>[2x]XKKLLKCLKCLLX

Herein we report the first X-ray crystal structures of mixed chirality α-helices in short peptides comprising only natural residues as the example of a stapled bicyclic and a linear membrane disruptive amphiphilic antimicrobial peptide (AMP) containing seven l- and four d-residues, as complexes of fucosylated analogs with the bacterial lectin LecB. The mixed chirality α-helices are superimposable onto the homochiral α-helices and form under similar conditions as shown by CD spectra and MD simulations but non-hemolytic and resistant to proteolysis. To get a direct insight into the structure of AMBP bp65/bp69 and their linear analogs ln65/ln69, we performed several crystallization studies using either the compounds themselves or their racemates to be crystallized as pure compounds, or their fucosylated derivatives of both mirror image peptides as complexes with the P. aeruginosa lectin LecB. While previous reports of similar mixed chirality AMPs concluded on either unordered conformations or helical conformations appearing in a membrane environment based on deconvolution of FTIR spectra, here we reported X-ray crystallographic evidence of short mixed chirality helices consisting of only natural residues existing as helix bundles within the protein environment of a lectin and almost perfectly superimposable with their parent homochiral α-helices. These direct observations unequivocally demonstrate that the α-helical fold with only natural residues can sometimes tolerate multiple stereochemical inversions without significant conformational changes.

Herein we report that optimization of bp3 by sequence and residue chirality variations followed by structural studies led us to the first X-ray crystal structure of an AMPB in the form of bp65. The structure of bp65 features an α-helical fold essentially identical to that of the corresponding linear peptide ln65 but comprising a bicyclic helix staple. In all four individually resolved homochiral bicyclic structures, the peptides were present in almost perfectly superimposable conformations featuring nine of the eleven residues forming two full turns of a right-handed α-helix including the pair of stapling cysteines (ESI†). The two N-terminal residues and the N-terminal toluoyl double staple formed a turn conformation. In all four cases the α-helical fold resulted in an amphiphilic arrangement of hydrophobic and cationic residues corresponding to the helix-wheel model and explaining the membrane disruptive activities discussed above. Remarkably, the ten crystallographically non-equivalent stapled bicyclic α-helices observed in the X-ray structures of the homochiral rac-bp65 and bp70, and the mixed chirality bp71·LecB complex were essentially superimposable, with RMSD < 0.6 Å for the peptide backbones. In the case of bp65, bp71 and Fln65 the peptides were aggregated in bundles of four of more helices via hydrophobic contacts between leucine side chains.beta-D-threo-hexo-2,4-diulo-2,5-furanose | C6 H10 O6 | 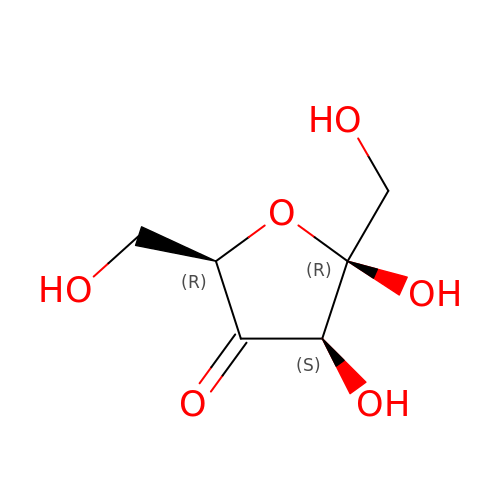LAWYCIPOFYQBDZ-PQLUHFTBSA-N> MGSDKIHHHHHHENLYFQGMKTIVIEDKQRIESIILQADACFVGITDLEGNPYVVPMNFGYENDTLYLHSGPEGGKIEMLQRNNNVCITFSLGHKLVYQHKQVACSYSMRSE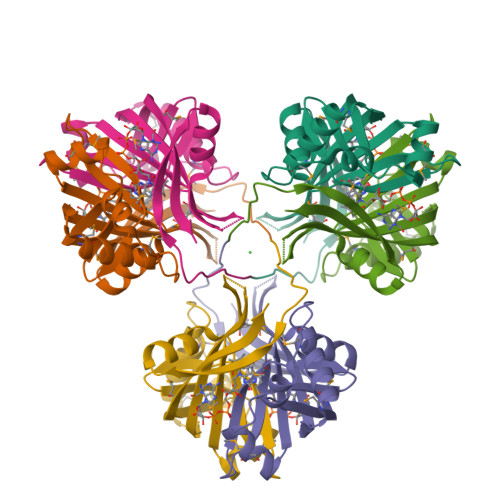SAMCRGKVEFIEDMEEKRHALDIIMRHYTKDQFSYSDPAVRNVKVWKVPVDQMTGKVFGLRADEKP>[2x]MATGIVKWF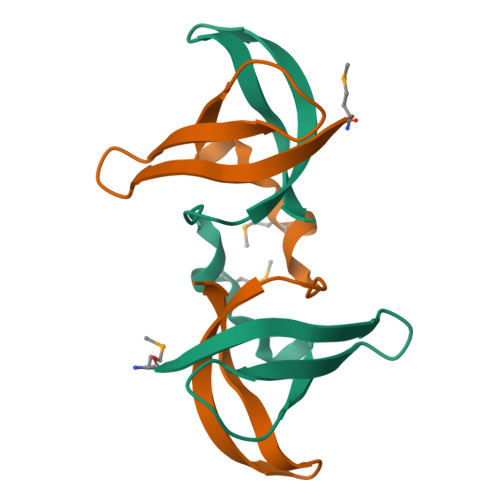NDAKGFGFITPDEGGEDLFAHFSAINMEGFKTLKEGQRVSFDVTTGPKGKQAANIQAA> GP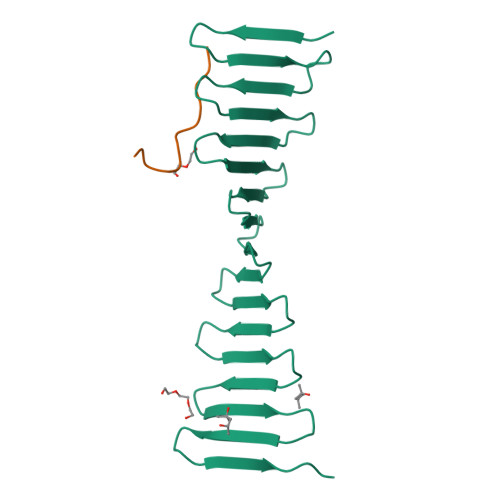LGSDSKIEKMLPDGGRLVVFPNGTRKELSADGQTVKVMFFNGDVKHTMPDQRVIYYYAEAQTTHITYPDGMEVLQFPNNQTEKHFPDGRKEITFPDQTVKTLHPDGREESVLTDGTIIQLNPDGSKVIQFNTGQREIHTADFKRREYPDGTVKTVYSDGRQETQYPTGRVRLKDPQGKVIMD;> DLSPRPSPNPHPVSQ> S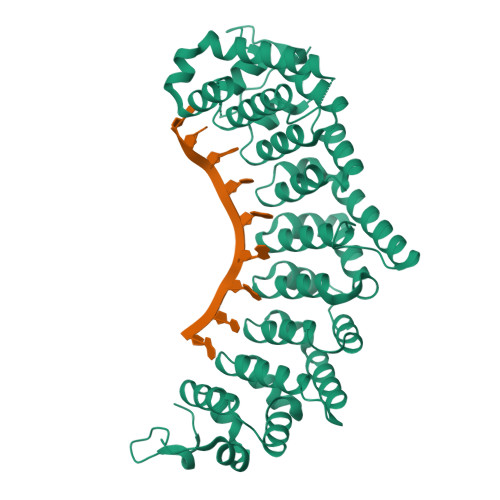SNNVLPTWSLDSNGEMRSRLSLSEVLDSGDLMKFAVDKTGCQFLEKAVKGSLTSYQKFQLFEQVIGRKDDFLKLSTNIFGNYFVQEIIGMSLTTYDDDNIKRQEKLKNFISSQMTDMCLDKFACRVIQSSLQNMDLSLACKLVQALPRDARLIAICVDQNANHVIQKVVAVIPLKNWEFIVDFVATPEHLRQICFDKYGCRVVQTIIEKLTADSINVDLTSAAQHLRERALQRLMTSVTNRCQELATNEYANYIIQHIVSNDDLAVYRECIIEKCLMRNLLSLSQEKFASHVVEKAFLHAPMELLAEMMDEIFDGYMPHPGTGKDALDIMMFHQFGNYVVQCMLTICCDAVSGRRQTKEGSYDHANSFQVWLKKLHSRVTKERHRLSRFSSGKKMIETLAHLRSTHPIYGLQSSGHESFKTDCFSTASEHDGLELEKNGIEEGNLRLMRTFSP>AIADFFPPHLLKKVVSEVVATFLLVFMTCGAAGISGSDLSRISQLGQSIAGGLIVTVMIYAVGHISGAHMNPAVTLAFAVFRHFPWIQVPFYWAAQFTGAICASFVLKAVIHPVDVIGTTTPVGPHWHSLVVEVIVTFNMM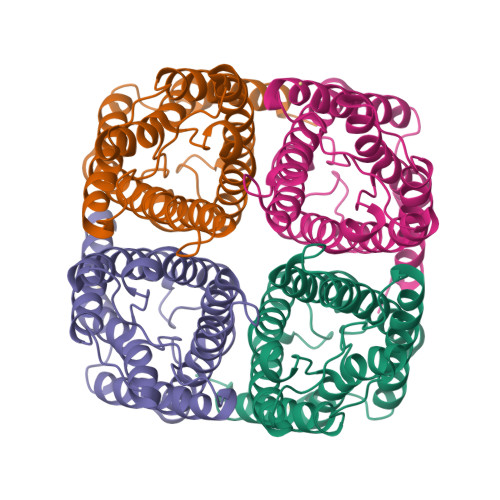FVTLAVATDTRAVGELAGLAVGSAVCITSIFAGAISGGSMNPARTLGPALASNKFDGLWIYFLGPVMGTLSGAWTYTFIRFEDTPK[8x]> MTMGSSHHHHHHSSGRENLYFQGHMAARSAPSPAGAPRPGLRERKKTRTREAIRAATYGLIRQQGYEATTVEQIAERAEVSPSTVLRYFPTREDIVLTDEYDPVMAAELAARPAGEPWSDSLRHVLRKALGLGAGEEAELIRLRTRLL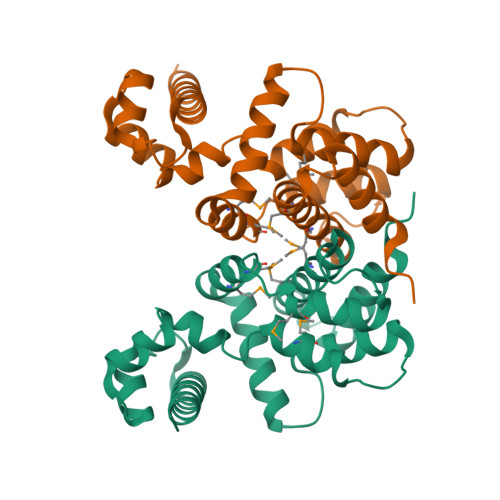AEVPAVRARMLENMSDTGRMLARAIADRTGLDPDGLEVRIVSMSLVGGLMEVSRYWAEHDHEESLAELVDRALDALENGLPALRESDRESDREGDRGGHREDRREGPRKDGS>MGSSHHHHHHSQDPMSLIKKKNKDIRIIPLGGVGEIAKNMYIVEVDDEMFMLDAGLMFPEDEMLGVDIVIPDIQYVIENKERLKGIFLTHGHEHAIGAVSYVLEQIDAPVYGSKLTIALVKEAMKARNIKKKVRYYTVNHDSIMRFKNVNVSFFNTTHSIPDSLGVCIHTSYGSIVYTGEFKFDQSLHGHYAPDLKRMAEIGDEGVFALISDSTEAEKPGYNTPENIIEHHMYDAFAKVKGRLIVSCYASNFVRIQQVLNIASQLNRKVSFLGRSLESSFNIARKMGYFDIPKDLLIPINEVENYPKNEVIIIATGMQGEPVEALSQMARKKHKIMNIEEGDSIFLAITASANMEVIIADTLNELVRAGAHIIPNNKKIHASSHGCMEELKMMLNIMKPEYFVPVQGEF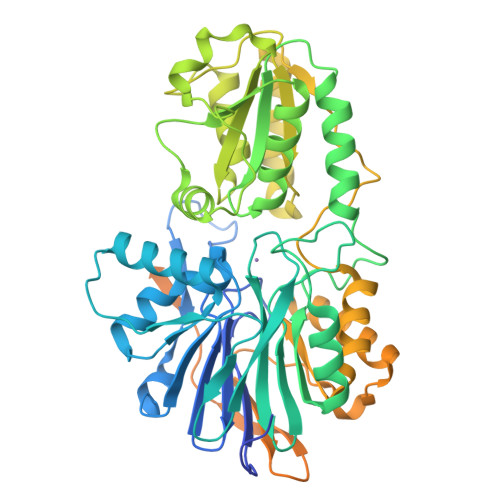KMQIAHAKLAAETGVAPEKIFLVEKGDVISYNGKDMILNEKVQSGNILIDGIGVGDVGNIVLRDRHLLAEDGIFIAVVTLDPKNRRIAAGPEIQSRGFVYVRESEELLKEAEEKVRKIVEEGLQEKRIEWSEIKQNMRDQISKLLFESTKRRPMIIPVISEI[4x]>[4x]GPGSQRQFARVKLPARIRYIGANREGVDARLLDLSAGGFAFTASGAPIQP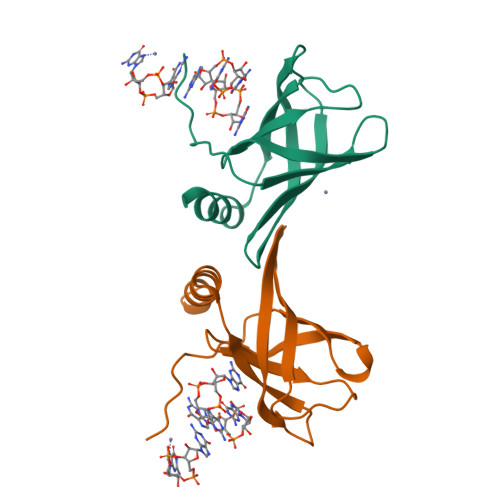GDLYKGKLLFQVDSISFSLEVEFQVRSVDPASRRVGCEFQNLKPREVAALRYLITSYLAGE N-(4-((2-fluorophenyl)(hydroxy)methyl)phenyl)acetamide 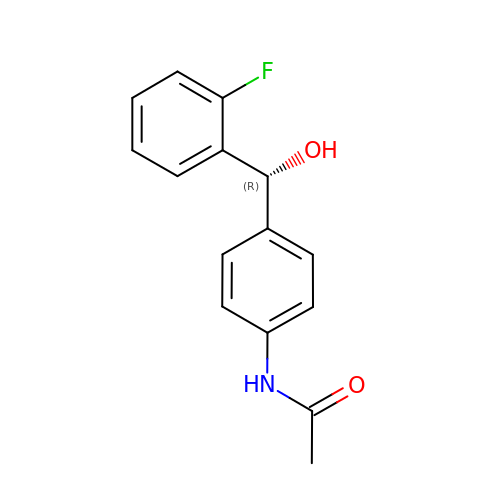| C15 H14 F N O2 | FGVHLIFJYKZKOI-OAHLLOKOSA-N> DRHHHHHHKLSTPGPPLFNVSLDVAPELRWLPVLRHYDVELVRAAVAQVIG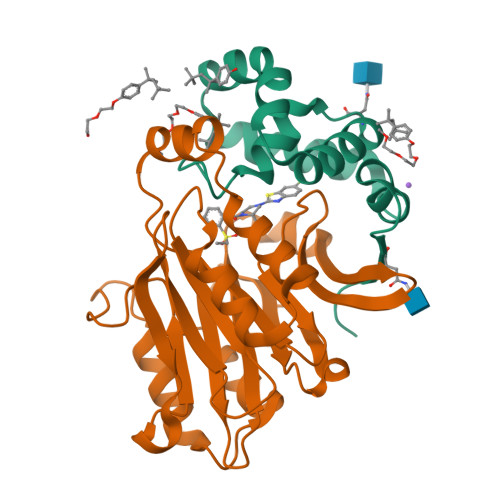DRVPKWVLALIEKGALKLERLLPPPFTAEIRGMCDFLNLSLADGLLVNLAYEYSAF;> CTSIVAQDSRGHVYHGRNLDYPYGSILRKLTVDVQFLKNGQIAFTGTTFIGYVGLWTGQSPHKFTVSGDERDRGWWWENLVAALFLRHSPISWLLRTTLSEAESFEAAVYRLAKTPLIADVYYIVGGTNPREGVVITRNRDGPADIWPLDPLKGVWFLVETNYDHWKPAPEEDDRRTPAIKALNATGQAKLSLETLFQVLSVVPVYNNYTIYTTVMSAASPDKYMTRIRNPS>MAMSQQDLPTLFYSGKSNSAVPIISESELQTITAEPWLEISKKGLQLEGLNFDRQGQLFLLDVFEGNIFKINPETKEIKRPFVSHKANPAAIKIHKDGRLFVCYLGDFKSTGGIFAATENGD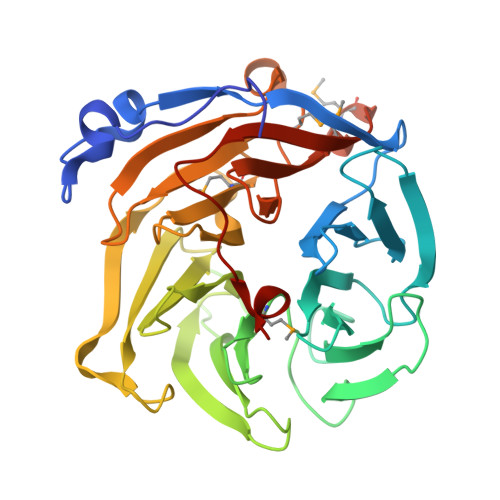NLQDIIEDLSTAYCIDDMVFDSKGGFYFTDFRGYSTNPLGGVYYVSPDFRTVTPIIQNISVANGIALSTDEKVLWVTETTANRLHRIALEDDGVTIQPFGATIPYYFTGHEGPDSCCIDSDDNLYVAMYGQGRVLVFNKRGYPIGQILIPGRDEGHMLRSTHPQFIPGTNQLIICSNDIEMGGGSMLYTVNGFAKGHQSFQFQLEHHHHHH[12x]>SNAMKDILRDIGVIARALDSISNIEFKELNLAKGQFIYLVRICENQGIIQEKLVDILKIDRTTASRAIKNLEKNGLIIKKQNKNNKKNKLLFPTEKGQQLYPLIIRENEYSNAVALKGFTEAEINMLTDALKKVKENIADDWLYVKKGNKRSY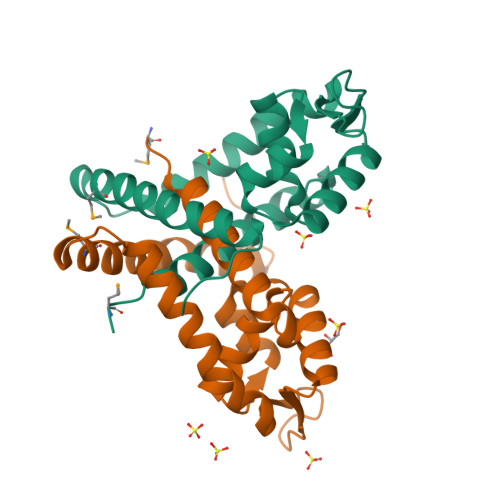[2x]As the multifunctional protein within the Flaviviridae family, Non-structural protein 1 (NS1) is considered as a promising target against flaviviruses. Moreover, the sNS1 lipoprotein is involved in virion production, immune evasion, and multiple aspects of pathogenesis. The NS1 monomer has 352 amino acids, forms 2 α-helices and 20 β-strands, and contains 12 conserved cysteine residues that form 6 intramolecular disulfide bonds. The NS1 monomer consists of three distinct domains: a β-roll domain (residues 1–29, β1–2), a wing domain (residues 38–151, β4–7 and α1–2), and a β-ladder domain (residues 181–352, β10–20). β3, β8, and β9 are from a ‘‘connector’’ domain (residues 30–37 and 152–180) and connect the wing to the β-roll and β-ladder domains.

Here, we observed that the recombinant sNS1 dimer from a YFV 17D strain exists in multiple-oligomeric states, predominantly in the tetrameric form. The final reconstruction of 215,543 particles yielded a structure (named YFV_NS1_tetramer) at a 3.57 Å resolution. The structure of the YFV_NS1_tetramer presents an asymmetrical “H” shape, which consists of two NS1 dimers (Aa and Bb) stacked through the inner hydrophobic surfaces. The distance between the centroids of Monomer A and B (42.5 Å) is smaller than the distance of Monomer a and b (54.6 Å). Thus, Monomer B leans towards Monomer A, while Monomer b extends outward. The buried interface area between dimer Aa and Bb is 853.7 Å2 via a PISA calculation. The tetrameric structure showed that the interface between dimer Aa and Bb is mainly contributed by the hydrophobic residues from the β-roll domains and greasy fingers. However, the DENV2 and ZIKV tetramers have a buried interface of ~650–690 Å2, which is much smaller than the one we observed in the YFV tetramer. These observations also indicate that the YFV tetramer is in a conformation that is distinct from the loose tetramer and stable tetramer. Therefore, we define this structure as a “semi-stable” tetramer, which may represent the intermediated state between the stable tetramer and the loose tetramer. Moreover, we also found the YFV tetramer to have multiple conformations, suggesting that the assembly of the YFV tetramer is flexible and that it has the potential to shift between stable tetramer and loose tetramer states.

>[4x]DQGCAINFGKRELKCGDGIFIFRDSDDWLNKYSYYPEDPVKLASIVKASFEEGKCGLNSVDSLEHEMWRSRADEINAIFEENEVDISVVVQDPKNVYQRGTHPFSRIRDGLQYGWKTWGKNLVFSPGRKNGSFIIDGKSRKECPFSNRVWNSFQIEEFGTGVFTTRVYMDAVFEYTIDCDGSILGAAVNGKKSAHGSPTFWMGSHEVNGTWMIHTLEALDYKECEWPLTHTIGTSVEESEMFMPRSIGGPVSSHNHIPGYKVQTNGPWMQVPLEVKREACPGTSVIIDGNCDGRGKSTRSTTDSGKVIPEWCCRSCTMPPVSFHGSDGCWYPMEIRPRKTHESHLVRSWVTAHHHHHH> ANGTSSAFTQIDNFSHF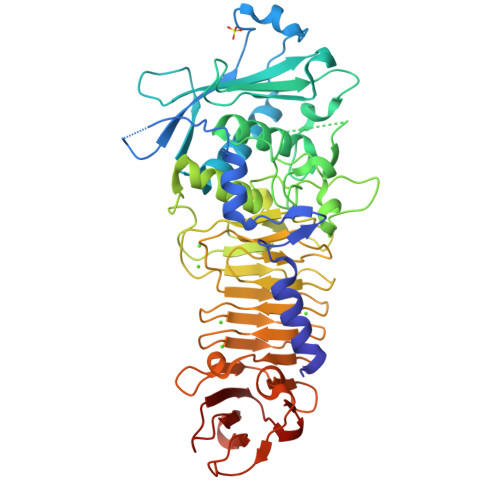YDRGDHLVNGKPSFTVDQVADQLTRSGASWHDLNNDGVINLTYTFLTAPPVGYASRGLGTFSQFSALQKEQAKLSLESWADVAKVTFTEGPAARGDDGHMTFANFSASNGGAAFAYLPNSSRKGESWYLINKDYQVNKTPGEGNYGRQTLTHEIGHTLGLSHPGDYNAGNGNPTYRDAVYAEDTRAYSVMSYWSEKNTGQVFTKTGEGAYASAPLLDDIAAVQKLYGANLETRADDTVYGFNSTADRDFYSATSSTDKLIFSVWDGGGNDTLDFSGFSQNQKINLTAGSFSDVGGMTGNVSIAQGVTIENAIGGSGNDLLIGNDAANVLKGGAGNDIIYGGGGADVLWGGTGSDTFVFGAVSDSTPKAADIIKDFQSGFDKIDLTAITKLGGLNFVDAFTGHAGDAIVSYHQASNAGSLQVDFSGQGVADFLVTTVGQVATYDIVA> GPMKASLTFSLSGIYAPCSISRDIYLEYGDKKAECLYGTIRLPQYGPGCTPGKIVHCVLDDSLPFCSIVVPSKLFGFMPTQPTMDFCYFEPILDNVVPVLDSVTFLINEQLYSKLMDLPQEMQQIQFLHYKYNINSMETVVHSRDILTSGLCQILNCSPFPQGLVDFTETQLILVNDTEQKLSALK

The heterohexameric ATPases associated with diverse cellular activities (AAA)-ATPase Pex1/Pex6 is essential for the formation and maintenance of peroxisomes. Pex1/Pex6, similar to other AAA-ATPases, uses the energy from ATP hydrolysis to mechanically thread substrate proteins through its central pore, thereby unfolding them. Pex1 and Pex6 belong to a family of type 2 ATPases associated with diverse cellular activities (AAA)-ATPases that form hexameric complexes consisting of two stacked ATPase rings, D1 and D2, topped by N-terminal domains. Unlike these better-studied homohexameric AAA-ATPases, Pex1 and Pex6 form a heterohexameric ATPase with alternating Pex1 and Pex6 subunits.

To structurally characterize the Pex6 N1 domain, we first used limited proteolysis to determine the boundary of the domain to be amino acids 1 to 184. We recombinantly expressed and crystallized Pex6 1-184 and collected X-ray diffraction data to a resolution of 1.9 Å. We then used molecular replacement with an AlphaFold atomic model to determine the structure of the Pex6 N1 domain. The Pex6 N1-domain consists of two subdomains: a double-psi β barrel in the N-terminal half (N1a) followed by an α/ β roll subdomain (N1b). An X-ray crystal structure of the isolated N1 domain from yeast Pex6 showed that despite limited conservation of primary sequence, this domain shares the conserved structure of the NSF and Cdc48 N terminal domains. Structure-based alignment of the Pex6 N1 domain and Cdc48 N domain shows that Pex6 N1 has more prominent loops in the N1a subdomain (arrows) and an altered position of the N1b helices (arrowheads). The Pex6 N1 domain surface is largely hydrophilic and has a negatively charged surface in the N1a subdomain and positively charged patch in the N1b subdomain. In addition to more highly conserved residues in the hydrophobic core of the N1a and N1b subdomains, we observed conserved residues in the extended loops of the N1a subdomain (arrow) and a cluster of residues between the N1b helices that form a small hydrophobic patch (arrowhead). The atomic models derived from the crystal structure of the isolated Pex6 N1 domain aligned very well with the atomic model based on the cryo-EM map (RMSD 1.604). The biggest differences in the models were related to the loops with high B-factors in the crystal structure, which form the interface of the N1 domain with the N2 domain of Pex6.> MKPKRVQGKIVIEFPSEDIAEVVYTSVLY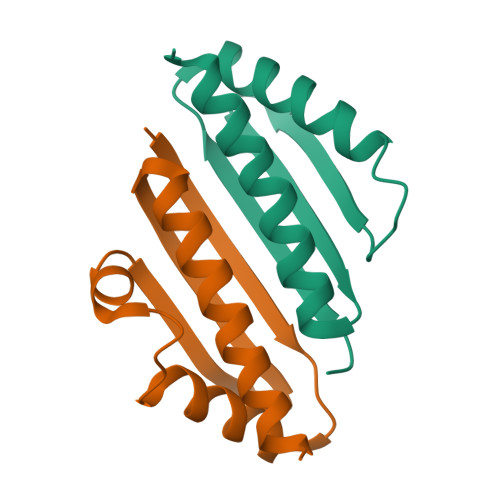EHVSVPYRRSRVNFRREGRRIVLEIEANDSSAMRGTVNSYLRWIKVALDVLNIHHHHHH;> MKIRAKVELTWEYEDEETAKAIANAVNVDNISIPEKLKKSLNLITFPDGARVVTKVKYEGEIESLVVALDDLIFAIKVAEEVLWSHPQFEK> HHHHHHPMSNTNIPTTENLYPEGAMVNKNKEGLNIDGKEVLAGSTNYYELTWDLDQYKGDKSSKEAIQNGFYYVDDYPEEALDVRPDLVKVADEKGNQVSGVSVQQYDSLEAAPKKVQDLLKKANITVKGAFQLFSADNPEEFYKQYVATG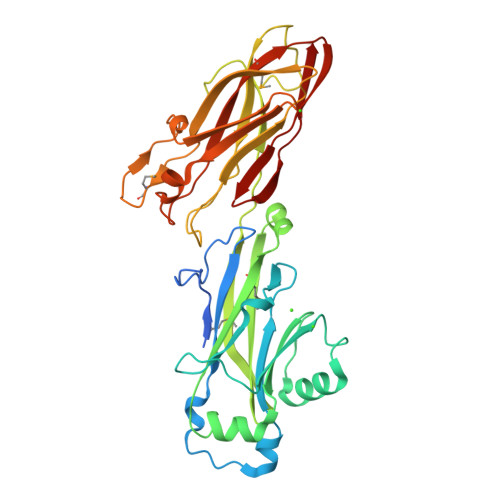TSLVITDPMTVKSEFGKTGGKYENKAYQIDFGNGYATEVVVNNVPKITPKKDVTVSLDPTSENLDGQTVQLYQTFNYRLIGGLIPQNHSEELEDYSFVDDYDQAGDQYTGNYKTFSSLNLTMKDGSVIKAGTDLTSQTTAETDATNGIVTVRFKEDFLQKISLDSPFQAETYLQMRRIAIGTFENTYVNTVNKVAYASNTVRTTT> GSHMSGWRLLLTRPDEECAALAASLGEAGVHSSSLPLLAIDPLEETPEQRTLMLDLDRYCAVVVVSKPAARLGLERLDRYWPQPPQQTWCSVGAATAAILEAYGLDVTYPEQGDDSEALLALPAFQDSLRVHDPKVLIMRGEGGREFLAERLRGQGVQVDYLPLYRRRAPDYPAGELLARVRAERLNGLVVSSGQGLQNLYQLAAADWPEIGRLPLFVPSPRVAEMARELGAQRVIDCRGASAPALLAALTSAA

Pseudomonas aeruginosa is a Gram-negative pathogen responsible for a significant level of hospital-acquired infections, particularly in burns victims and immunocompromised and cystic fibrosis patients. In an effort to accelerate early steps in drug discovery, the EU-funded AEROPATH project aims to identify novel targets in the opportunistic pathogen Pseudomonas aeruginosa by applying a multidisciplinary approach encompassing target validation, structural characterization, assay development and hit identification from small-molecule libraries. The crystal structures of eight of these targets, ranging from hypothetical unknown proteins to metabolic enzymes from different functional classes (PA1645, PA1648, PA2169, PA3770, PA4098, PA4485, PA4992 and PA5259), are reported here. The structural information is expected to provide a firm basis for the improvement of hit compounds identified from fragment-based and high-throughput screening campaigns.

Uroporphyrinogen III (U3) is the first cyclic tetrapyrrole compound in the haem-biosynthesis pathway and is located at a metabolic branching point. From U3, biosynthetic routes lead to haem, sirohaem or cobalamin (vitamin B12). The structure of P. aeruginosa uroporphyrinogen III synthase (HemD, PA5259) was solved to 2.4 Å resolution using Se-SAD phasing.> GGLEKDFLPLYFGWFLTKKSSETLRKAGQVFLEELGNHKAFKKELRHFISGDEPKEKLELVSYFGKRPPGVLHCTTKFCDYGKAAGAEEYAQQEVVKRSYGKAFKLSISALFVTPKTAGAQVVLTDQELQLWPSDLDKPSASEGLPPGSRAHVTLGCAADVQPVQTGLDLLDILQQVKGGSQGEAVGELPRGKLYSLGKGRWMLSLTKKMEVKAIFTGYYG

2′,3′-cyclic nucleotide 3′-phosphodiesterase (CNPase) comprises 4% of total myelin protein in the central nervous system (CNS), being the most abundant CNS non-compact myelin protein4. CNPase consists of an N-terminal polynucleotide kinase-like domain10, a catalytic phosphodiesterase domain11, and a membrane-anchored C-terminal tail, which contains a cysteine residue that undergoes isoprenylation. The catalytic domain enables the rapid hydrolysis of nucleoside 2′,3′-cyclic phosphates to nucleoside 2′-phosphates. The CNPase catalytic site, lying in a groove between two lobes, has pseudo two-fold symmetry and contains two apposing His-X-Thr-X (X denotes a hydrophobic residue) motifs, characteristic for 2H phosphoesterases 113537.

Additionally, we characterized the perdeuterated CNPase catalytic domain (dCNPcat) and determined its crystal structure at 1.04-Å resolution, allowing the observation of active site protonation states and dynamics, as well as water networks. Comparing the measured mass of dCNPcat in D2O (25976.0 Da) with the theoretical mass of 100% perdeuterated protein (26012.1 Da), the perdeuteration degree of dCNPcat was very high (97.9%). As the thin crystals of dCNPcat could not be grown to dimensions suitable for neutron diffraction, the structure was solved using X-ray crystallography and refined to an atomic resolution of 1.04 Å. This is by far the highest resolution obtained for CNPase so far. The proposed catalytic mechanism for CNPase involves two histidine residues in the active site; His309 deprotonates and activates the nucleophilic water molecule, and His230 coordinates the leaving group and protonates it upon completion of the reaction. Examination of the electron density maps for these residues confirms that in the apo state, His309 is deprotonated and His230 protonated. The chain of 4 water molecules at the bottom of the active site is coupled to another group of 4 water molecules above them – representing a true apo active site, without any bound buffer components. The outcome of a more detailed analysis is surprising; out of the 4 water molecules at the bottom, the central ones have 5 coordination contacts, while both of the distal ones only have 4, in a classical tetrahedral setting. Anisotropic B factor refinement and alternative conformations reveal directional disorder in the vicinity of the catalytic cavity, for example concerning a number of aromatic residues. In the case of dCNPcat, the most drastic geometric outlier is Trp289, which is sandwiched through C-H…π interactions between Pro290 and Gly305.>[3x]MRLNDPVHYDGAWHVYKYSDVKHVLMNDKIFSSN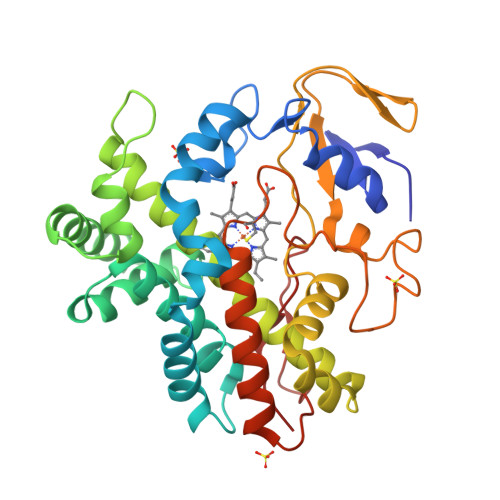PGNRYSNAGGISFITMDNPEHKEFRDISAPYFLPSKINDYKDFIEETSNDLIKNIDNKDIISEYAVRLPVNIISKILGIPDSDMPLFKLWSDYIIGNKRDENFNYVNNRMVSRLLEIFKSDSHGIINVLAGSSLKNRKLTMDEKIKYIMLLIIGGNETTTNLIGNMIRVIDENPDIIDDALKNRSGFVEETLRYYSPIQFLPHRFAAEDSYINNKKIKKGDQVIVYLGSANRDETFFDEPDLFKIGRREMHLAFGIGIHMCLGAPLARLEASIALNDILNHFKRIKIDYKKSRLLDNKMVLGYDKLFLS Here, we have sought to generate high-resolution crystallographic structures of the cellular interacting fiber-knob domains of species D adenoviruses HAdV-D26 and HAdV-D48. The fiber-knob is the receptor interacting domain of the fiber protein, one of three major capsid proteins along with the hexon and penton base, as shown schematically in Fig. 1a. We next calculated the amino acid variability at each position in the aligned adenoviral fiber-knob sequences, which revealed regions of broad conservation corresponding to β-strands which make up the main fold of the fiber-knob trimer. Each monomer interacts with two neighbouring copies to form a homotrimer with 3-fold symmetry and a highly stable interface. Analysis of the adenovirus loops reveals an intricate network of polar interactions which stabilise their three-dimensional structures.

The shorter HAdV-C5K DG loop does not clash with the CAR-D1 surface, whereas the extended HAdV-D26K DG loop forms a partial steric clash, with surface seen to clash with the aligned CAR-D1, and HAdV-D48K DG loop is seen to form an even larger steric clash. Our modelling studies indicate that the longer, inflexible DG loop of HAdV-D48K would be likely to sterically hinder the HAdV-D48K: CAR interaction at the β-interface to a greater extent than the more modest inhibition of the smaller and more labile loop of HAdV-D26K, which in turn would exhibit more inhibition of CAR binding than that of HAdV-C5K, where no steric inhibition is observed. SPR analysis indicates that HAdV-C5K binds strongly to CAR with a KD of 0.76 nM. While the KOff of the three fiber knob proteins are similar, the KOn is fastest for HAdV-C5K, with HAdV-D26K KOn being slower, and HAdV-D48K exhibiting the slowest KOn. The IC50 (the concentration of protein required to inhibit 50% of antibody binding) of HAdV-C5K is 7.0 ng/105 cells, while HAdV-D26K and HAdV-D48K demonstrate IC50 values 15.7 and 480 times higher at 0.110 μg/105 cells and 3.359 μg/105 cells, respectively, reflecting their reduced ability to engage CAR. While still low compared to the known CD46 interacting HAdV-B11K and HAdV-B35K binding energies, that for HAdV-C5K was higher than expected for a known non-CD46 interacting adenovirus. Inspection of the model shows that this is due to the close proximity of the large HAdV-C5 HI loop to CD46. The residues involved in the predicted interaction are not conserved in any known CD46 interface and suggesting these are random interactions. Furthermore, interaction between the DG loop and CD46 is integral to known CD46 binding interfaces and is prevented by the HAdV-C5K HI loop laying between them.

>[2x]NDKLTLWTTPAPSPNCRLNAEKDAKLTLVLTKCGSQILATVSVLAVKGSLAPISGTVQSAHLIIRFDENGVLLNNSFLDPEYWNFRNGDLTEGTAYTNAVGFMPNLSAYPKSHGKTAKSNIVSQVYLNGDKTKPVTLTITLNGTQETGDTTPSAYSMSFSWDWSGHNYINEIFATSSYTFSYIAQE;> KNNDKLTLWTTPAPSPNCRLNAEKDAKLTLVLTKCGSQILATVSVLAVKGSLAPISGTVQSAHLIIRFDENGVLLNNSFLDPEYWNFRNGDLTEGTAYTNAVGFMPNLSAYPKSHGKTAKSNIVSQVYLNGDKTKPVTLTITLNGTQETGDTTPSAYSMSFSWDWSGHNYINEIFATSSYTFSYIAQE> EQGNRPVETENIARGKQASQSSTAHGGAATRAVDGNVDSDYGHHSVTHTNFEDNA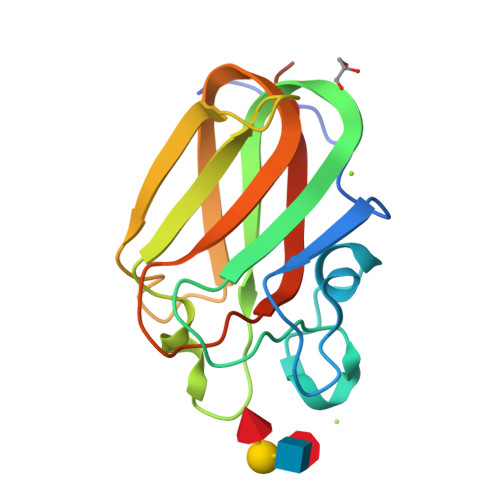WWQVDLGKTENVGKVKLYNRGDGNVANRLSNFDVVLLNEAKQEVARQHFDSLNGKAELEVFFTAKDARYVKVELKTKNTPLSLAEVEVFRSATTQVGC>[2x]MQVKPCTPEFYQTHFQLAYRLQSRPRGLALVLSNVHFTGEKELEFRSGGDVDHSTLVTLFKLLGYDVHVLCDQTAQEMQEKLQNFAQLPAHRVTDSCIVA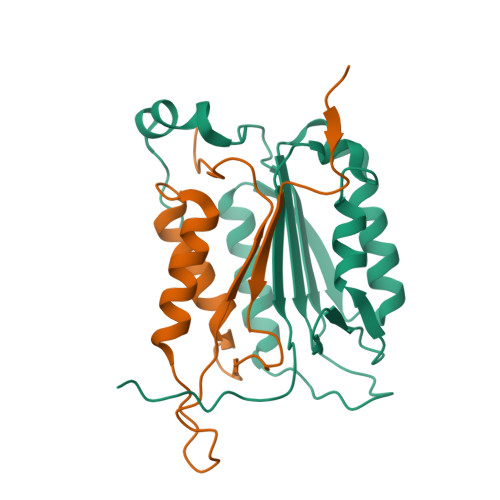LLSHGVEGAIYGVDGKLLQLQEVFQLFDNANCPSLQNKPKMFFIQACRGDETDRGVDQQD;>[2x]GKEKLPKMRLPTRSDMICGYACLKGTAAMRNTKRGSWYIEALAQVFSERACDMHVADMLVKVNALIKDREGYAPGTEFHRCKEMSEYCSTLCRHLYLFPGHPPTLEHHHHHH>[2x]HHHHHHLAYSLDATASFLNFVSSKKTHVLETHRFDVLSGGISTAG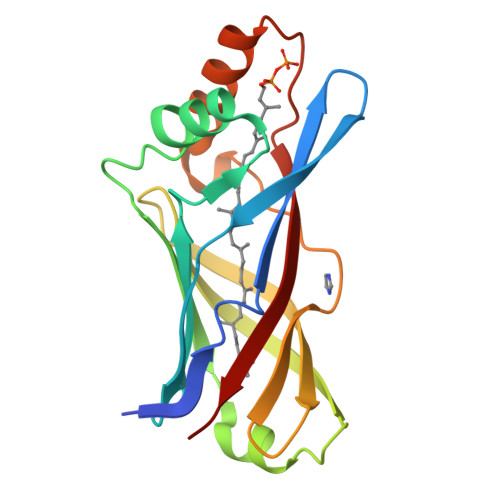EAQLVIDLNSVNTGIDVRNGRMRDYLFETATYSVATVTVPVDLAAVAGLAVGEDMLVDVSATLDLHGVPGVIDTQLNVQRLSATRIMVQNQSPLLIKAADYSLEAGIETLRNLASLNVISTTVPVDFVLFYEAP>GSAENESTPIQQLLEHFLRQLQRKDPHGFFAFPVTDAIAPGYSMIIKHPMDFGTMKDKIVANEYKSVTEFKADFKLMCDNAMTYNRPDTVYYKLAKK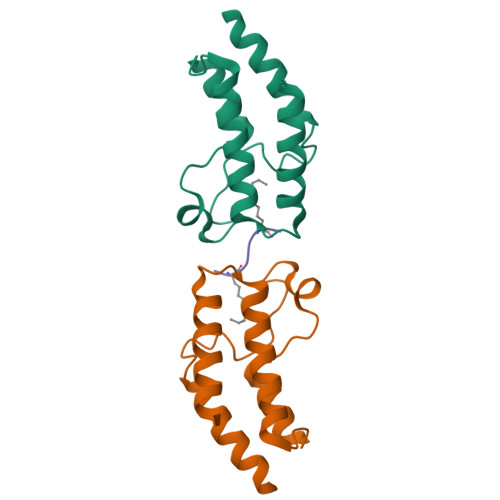ILHAGFKMMSK[4x];>[2x]SGRGXGGXGLG> DLFTLSFSPDLSIASEAEQLTLQSKDDRLILEHPQPGLRTALEQLKQGNLTLAQLTELV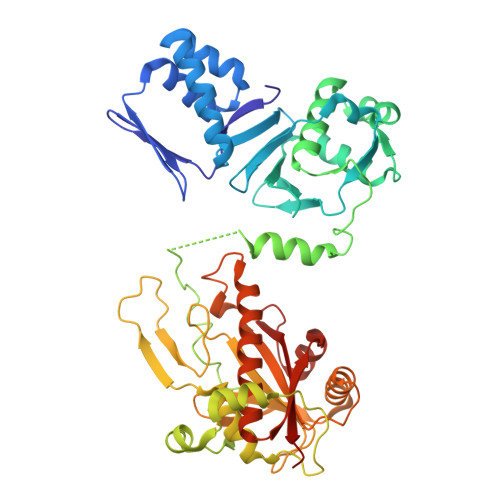SEQDGVEAGITFASELEKLVDLGWICHSVLPLITAIPIAKDYELNVPDSSWQTTAIALSRFAFLHQDLQQLVLESPRSKSKLVILDWRVGAVIAKLAQSDRGFIFATSADSLLADLSLELEELKRLFALLIATQMMDLEPEDETITQWKFHNLLFHHYTRLGRLDNSRKLNLPVFEHRDRYPYVKPVISTQAIPLVKPDLTALATTDMTLTEAIETRRSIREYSDQPITLAQLGEFLYRCARVKAVYTLPEDPMQVGESTTRPYPSGGALYELEIYPLVHQCGDLAAGLYHYQPLSHTLHPVADWTPEVESLVYDAWRATGQQSIPQIVLIITARFGRLFWKYHDIAYSLILKHVGVLYQTFYLVATAMQLAPSAIGAGNTTKFCQIAGLNPDEEASVGEFSLGAAKP> GPAMLPISMSDEGDSFLVKDSIGENKIPKNPSKVVIL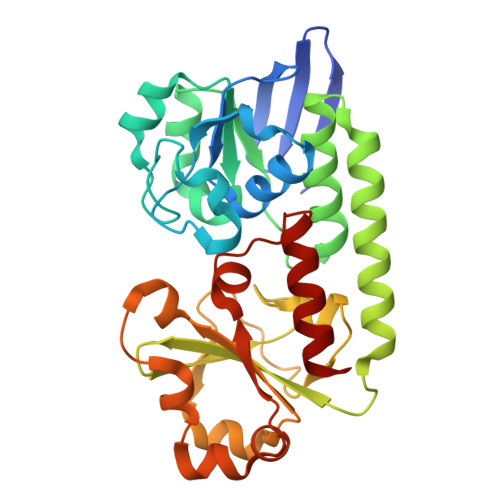DLGILDTFDALKLNDKVVGVPAKNLPKYLQQFKNKPSVGGVQQVDFEAINALKPDLIIISGRQSKFYDKLKEIAPTLFVGLDNANFLSSFENNVLSVAKLYGLEKEALEKISDIKNEIEKAKSIVDEDKKALIILTNSNKISAFGPQSRFGIIHDVLGINAVDENIKVGTAGKSINSEFILEKNPDYIFVVDRNVILGNKERAQGILDNALVAKTKAAQNKKIIYLDPEYWFLASGNGLESLKTMILEIKNAVK> MAELIPVENLDVVKAIVAEHREVPGCLMQILQETQLKYGYLPLELQGTIADELGIPLTEVYGVATFYSQFTLKPKGKYKIGICLGTACYVRGSQAIIDKVNSVLGTQVGDTTEDGKWSV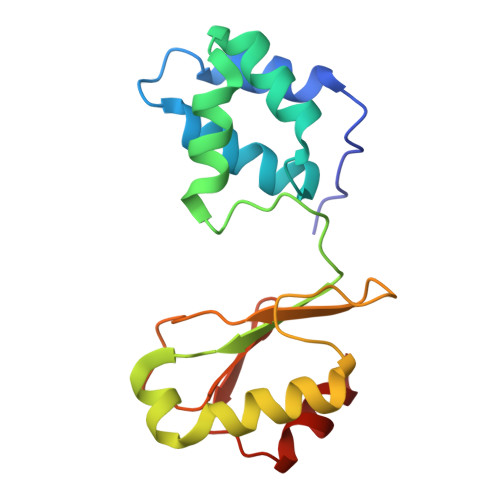DATRCVGACGLAPVMMINEEVFGRLTVDEIPGILEKY>AEPVYPDQLRLFSLGQGVCGDKYRPVNREEAQSVKSNIVGMMGQWQISGLANGWVIMGPGYNGEIKPGTASNTWCYPTNPVTGEIPTLSALDIPDGDEVDVQWRLVHDSANFIKPTSYLAHYLGYAWVGGNHSQYVGEDMDVTRDGDGWVIRGNNDGGCDGYRCGDKTAIKVSNFAYNLDPDSFKHGDVTQSDRQLVKTVVGWAVNDSDTPQSGYDVTLRYDTATNWSKTNTYGLSEKVTTKNKFKWPLVGETELSIEIAANQSWASQNGGSTTTSLSQSVRPTVPARSKIPVKIELYKADISYPYEFKADVSYDLTLSGFLRWGGNAWYTHPDNRPNWNHTFVIGPYKDKASSIRYQWDKRYIPGEVKWWDLNWTIQQNGLSTMQNNLARVLRPVRAGITGDFSAESQFAGNIEIGAPVPLAADSKVR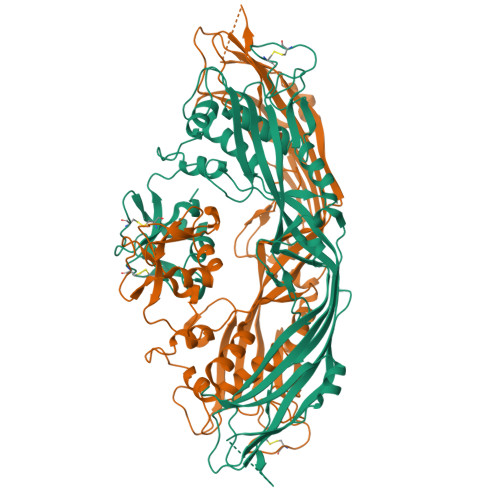RARSVDGAGQGLRLEIPLDAQELSGLGFNNVSLSVTPAANQ[2x]> ESYLSPAQSVKPKINTEEKLPREKLNPPTPSIYLESKRDAFSPVLLQFCTDPRNPITVIRGLAGSLRLNLGLFSTKTLVEASGEHTVEVRTQVQQPSDENWDLTGTRQIWPCESSRSHTTIAKYAQYQASSFQESLQEELEVLFQGPTKAARKSAPATGGGSSGSHHIIKFGTNIDLSDAKRWKPQLQELLKLPAFMRVTSTGNML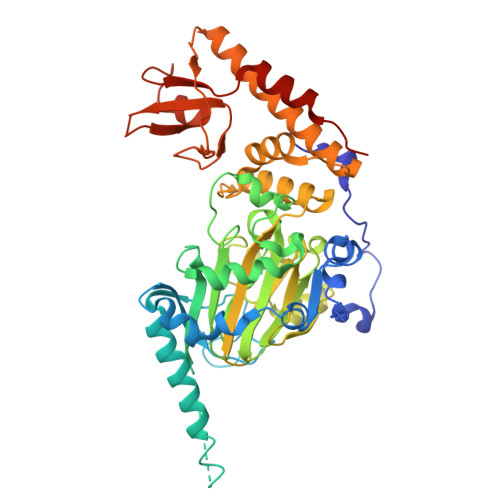SHVGHTILGMNTVQLYMKVPGSRTPGHQENNNFCSVNINIGPGDCEWFAVHEHYWETISAFCDRHGVDYLTGSWWPILDDLYASNIPVYRFVQRPGDLVWINAGTVHWVQATGWCNNIAWNVGPLTAYQYQLALERYEWNEVKNVKSIVPMIHVSWNVARTVKISDPDLFKMIKFCLLQSMKHCQVQRESLVRAGKKIAYQGRVKDEPAYYCNECDVEVFNILFVTSENGSRNTYLVHCEGCARRRSAGLQGVVVLEQYRTEELAQAYDAFTLAPASTSR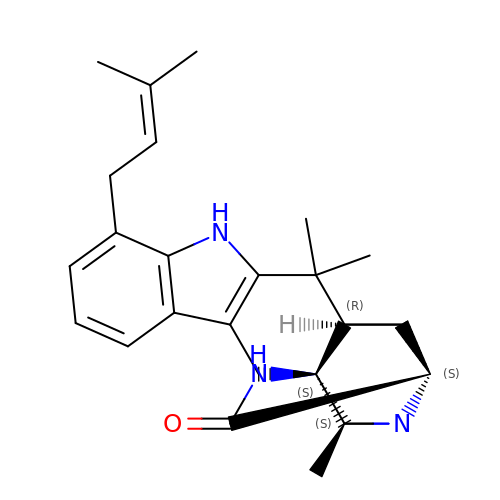(6aR,7aS,11S,13aS)-6,6,11-trimethyl-4-(3-methylbut-2-en-1-yl)-6,6a,7,8,9,10,11,14-octahydro-5H,13H-13a,7a-(epiminomethano)quinolizino[2,3-b]carbazol-16-one | C28 H37 N3 O | OMTRTWVJZBEAAJ-AEQSLLNGSA-N pmcCRISPR-associated transposons (CASTs) have co-opted Cas genes for RNA-guided DNA integration and are promising candidates for novel genome-editing methods. Despite remarkable diversity, all RNA-directed transposition systems characterized to date share multiple components: a CRISPR effector (Cas12k or Cascade), proteins dedicated to target capture (TniQ + TnsC), and a transposase called TnsB. By analogy to work from prototypic Tn7 (2), TnsB carries out transposon end recognition, pairing, and the chemical steps which result in integration of cognate element DNA. We determine the molecular mechanism of TnsB recruitment to the target site (via the AAA+ regulator TnsC) and the structural details of the TnsB transposase.

To understand how TnsB recognizes and pairs the transposon ends and subsequently juxtaposes them to target DNA, we reconstituted and imaged a TnsB strand-transfer complex (STC) using a symmetric DNA substrate containing the first 45 bp of the ShCAST transposon’s left end. Reconstitution with this substrate resulted in a homogeneous, stable assembly (as assessed by size-exclusion chromatography) with which we obtained a high-resolution cryo-electron microscopy (cryo-EM) reconstruction (3.7-Å global resolution). TnsB forms a C2-symmetric tetrameric assembly organized around the strand-transfer DNA. The overall architecture and arrangement of functional domains are remarkably similar to the MuA STC. B-L2 helix IIIα (red asterisk) wraps around the back of domain IIα of B-L1 (light purple) to nestle between the B-L1 (light purple and tan) subunits, forming interactions with both. The TnsB STC has highly distorted DNA (120° bend) surrounding the 5-bp target site (brown) comparable to MuA. Consistent with this, the DDE catalytic residues (D205, D287, and E321) are positioned at the target–donor junction precisely at the DNA distortion (red star), coordinating a magnesium ion with the scissile phosphate poised for nucleophilic attack. The linker connecting domains Iγ and IIα in the L1-bound TnsB subunit snakes underneath each 5′ end of the element in the nontransferred strand, forming stabilizing interactions with the first two nucleotide positions. We observe “melting” of the 5′ end of the nontransferred strand through a flipped-out base (T1). This specific conformation is stabilized by aromatic interactions with W178 and hydrogen bonding with S175 and R380.

>[4x]MNSQQNPDLAVHPLAIPMEGLLGESATTLEKNVIATQLSEEAQVKLEVIQSLLEPCDRTTYGQKLREAAEKLNVSLRTVQRLVKNWEQDGLVGLTQTSRADKGKHRIGEFWENFITKTYKEGNKGSKRMTPKQVALRVEAKARELKDSKPPNYKTVLRVLAPILEKQQKAKSIRSPGWRGTTLSVKTREGKDLSVDYSNHVWQCDHTRVDVLLVDQHGEILSRPWLTTVIDTYSRCIMGINLGFDAPSSGVVALALRHAILPKRYGSEYKLHCEWGTYGKPEHFYTDGGKDFRSNHLSQIGAQLGFVCHLRDRPSEGGVVERPFKTLNDQLFSTLPGYTGSNVQERPEDAEKDARLTLRELEQLLVRYIVDRYNQSIDARMGDQTRFERWEAGLPTVPVPIPERDLDICLMKQSRRTVQRGGCLQFQNLMYRGEYLAGYAGETVNLRFDPRDITTILVYRQENNQEVFLTRAHAQGLETEQLALDEAEAASRRLRTAGKTISNQSLLQEVVDRDALVATKKSRKERQKLEQTVLRSAAVDESNRESLPSQIVEPDEVESTETVHSQYEDIEVWDYEQLREEYGF> MLKDFGKKIKSLRLEKGLTK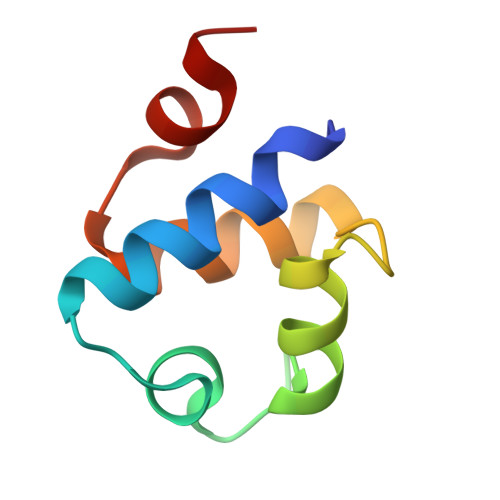EAVCLDESQLSTRQLTRIESGQSTPTLNKAVYIAGRLGVTLGYLTDGE>MAHGPFNAQGFTDFDSLS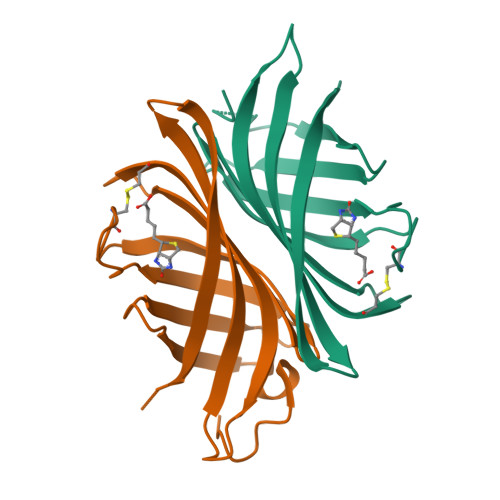GTSTTWVNELGSVMTIDVDRKGGVTGYYVNNAPGTGCRGLPYDLSGHAHGSTIAFSVVWSNGIADCRSATSWAGYARKTFGGGVQIVTQWSLAFVGKAGGKIETGQNVFTYQAYDAQPSPADK[4x]>NPYTIYPPVPKTASINGFADRIYDQIPKCAQECVKQSTSSTPCPYWDTGCLCVIPNFTGAVGNCVASKCRGADVTNFRKLAVGACAAAGVWDP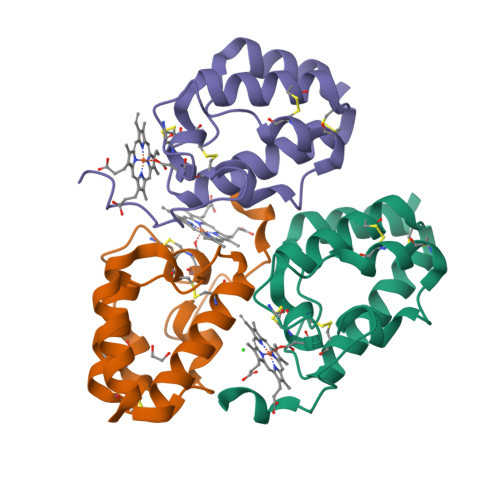YWIIPASVSSALDAAATA[3x]> VTNVGEDGEPGETEPRHALSPVDMHVHTDVSFLLDRFFDVETLELSNLTGSPATHVLDPFGSTAQLAWARLLNTCTYFFSDLELSIQFKFTTTPSSVGEGFVWVKWFPVGAPTKTTDAWQLEGGGNSVRIQQLAVAGMSPTVVFKIA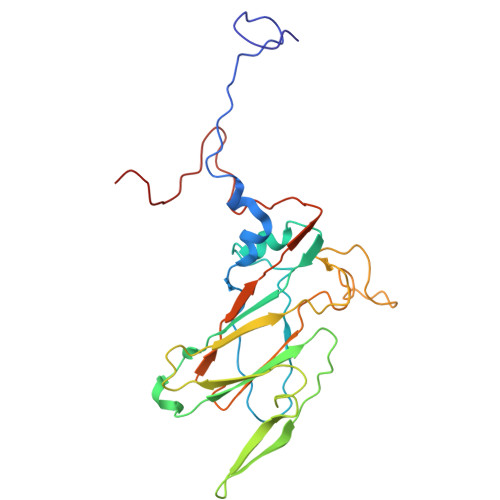GSRSQACGFSVPYTSMWRVVPVFYNGWGAPTKEKATYNWLPGAHFGSILLTSDAHDKGGCYLRYRFPRANMYCPRPIPPAFTRPADKTRHKFPTNINKQ>[6x]MRTLL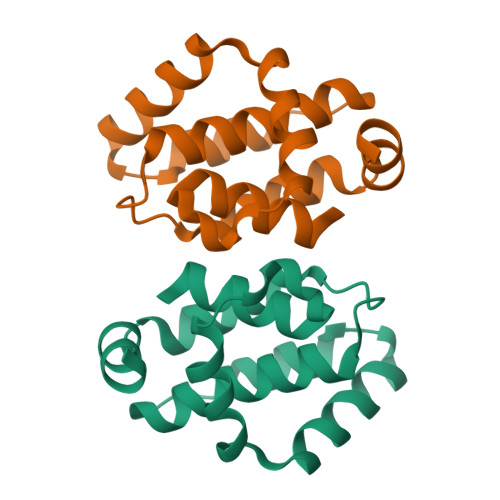IRYILWRNDNDQTYYNDDFKKLMLLDELVDDGDVSTLIKNMRMTLSDGPLLDYLNQPVNNIEDAKRMIAISAKVARDIGERSEIRWEESFTILFRMIETYFDDLMIDLYGEKLEHHHHHH>VIKTVLTYQLDGSNRDFNIPFEYLARKFVVVTLIGVDRKVLTINTDYRFATRTTISLTKAWGPADGYTTIELRRVTSTTDRLVDFTDGSILRAYDLNVAQIQTMHVAEEARDLTTDTIGVNNDGHLDARGRRIVNLANAVDDRD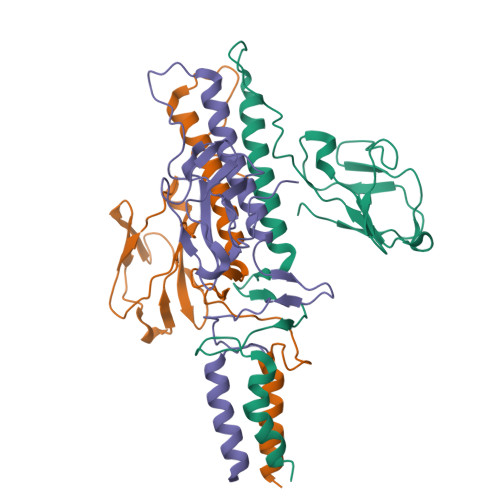AVPFGQLKTMNQNSWQARNE[3x]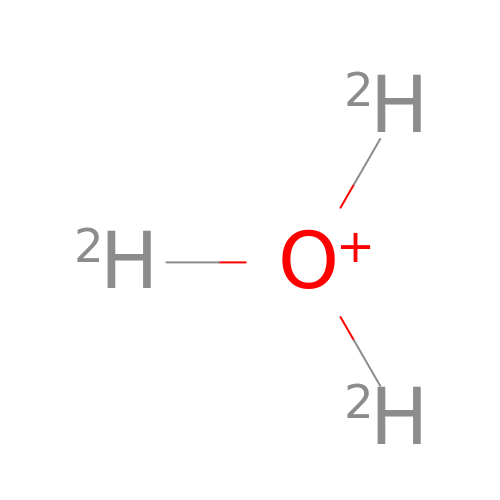trideuteriooxidanium | D3 O | XLYOFNOQVPJJNP-ZRLBSURWSA-O TGM6 is a natural antagonist of mammalian TGF-β signaling produced by the murine helminth parasite Heligmosomoides polygyrus. It differs from the previously described agonist, TGM1 (TGF-β Mimic-1), in that it lacks domains 1/2 that bind TGFBR1. It nonetheless retains TGFBR2 binding through domain 3 and potently inhibits TGF-β signaling in fibroblasts and epithelial cells, but does not inhibit TGF-β signaling in T cells, consistent with divergent domains 4/5 and an altered co-receptor binding preference. In this work, we show that TGM6, whose D3 shares 66% identity to TGM1-D3, binds TGFBR2, but does not bind TGFBR1 or other type I and type II receptors of the TGF-β family.

To identify the underlying molecular basis by which TGM6-D3 binds and recognizes TGFBR2, we isolated the TGM6-D3:TGFBR2 complex using size exclusion chromatography, screened for diffracting crystals, and determined the structure to a resolution of 1.40 Å. We found one TGM6-D3:TGFBR2 complex in the crystallographic asymmetric unit and interpretable density for residues 46–153 of TGFBR2 and residues 16–65 and 71–102 of TGM6-D3. There is a single large interface between TGM6-D3 and TGFBR2 with an area of 661 Å2. TGM6-D3 engages TGFBR2 primarily through the edge β-strand, β4, and does so through the interface near the C-terminus with the residues anticipated, Ile78 from β-strand 3, Tyr93 and Arg95 from β-strand 4, and Arg38 from the tip of the HVL27. The interface between TGM6-D3 and TGFBR2 is a remarkable mimic of the interface between TGF-β1/-β3 and TGFBR238,39, with a central hydrophobic region flanked by hydrogen-bonded ion-pairs at the periphery. On one side of the interface, TGFBR2 Asp55 and Glu78 form hydrogen-bonded ion-pairs with TGM6-D3 Arg95 and Arg38, respectively, the first of which closely mimics the interaction between TGFBR2 Asp55 and TGF-β1/-β3 Arg394. In the central hydrophobic region, TGFBR2 Ile76 inserts into a hydrophobic pocket formed by TGM6-D3 residues Ile78, Tyr80, and Tyr93, mimicking the interaction between TGFBR2 Ile76 and the hydrophobic pocket between the fingers of TGF-β formed by Trp332, Tyr390, and Val392. On the side of the interface opposite the TGM6-D3 Arg95:TGFBR2 Asp55 interaction, TGFBR2 Asp141 forms a hydrogen bond with the phenolic hydroxyl of TGM6-D3 Tyr80 and TGFBR2 Glu142 forms a hydrogen-bonded ion-pair with TGM6-D3 Arg82, mimicking the hydrogen-bonded ion-pair between TGFBR2 Glu142 and TGF-β1/-β3 Arg325. Though the overall architecture of the TGM6-D3:TGFBR2 interface is similar to the TGF-β1/-β3:TGFBR2 interface, it is about 50% larger (661 Å2 vs. 479 Å2 for the TGF-β1/-β3:TGFBR2 interface) and it has a greater number of hydrogen bond and ionic interactions.

> MVTDNNGAVKFPQLCKFCDVRFSTCDNQKSCMSNCSITSICEKPQEVCVAVWRKNDENITLETVCHDPKLPYHDFILEDAASPKCIMKEKKKPGETFFMCSCSSDECNDNIIFSEEYN;> GSGTGSSCPPLPDDETVWYEYYGYVDGRHTVGDAAIKDSLENYPPNTHARRHCKALSKKADPGEFVAICYQRRGTSESQWQYYPRIASCPDP> ADDIVLKAKNGDVKFP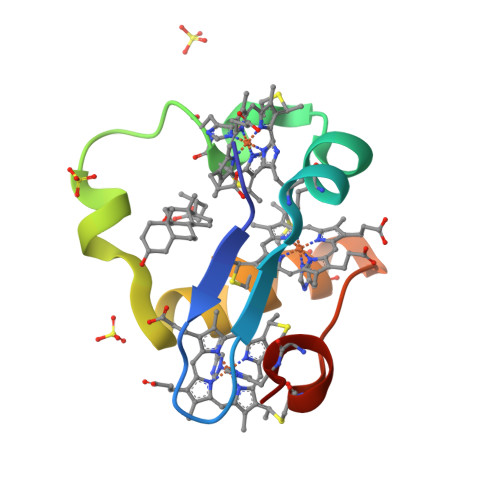HKAHQKAVPDCKKCHEKGPGKIEGFGKEMAHGKGCKGCHEESKKGPTKCGECHKK N-(4-{[4'-(carbamoylamino)-6-hydroxybiphenyl-3-yl]oxy}-3,5-dichlorophenyl)propanamide | C22 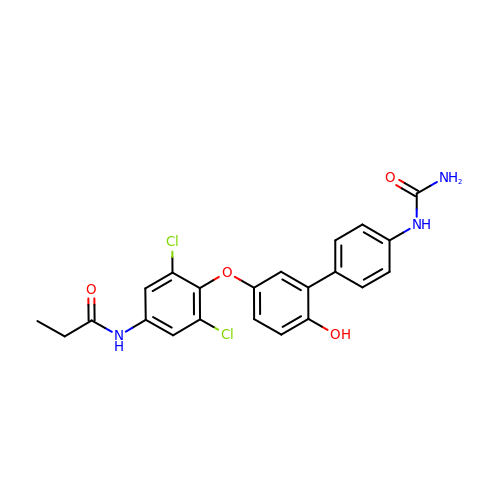H19 Cl2 N3 O4 | ULXKYEOCXYPCJV-UHFFFAOYSA-N We describe complex formation between a designed pentameric β-propeller and the anionic macrocycle sulfonato-calix[8]arene (sclx8), as characterized by X-ray crystallography and NMR spectroscopy. Each blade of this β-propeller is a 47-residue monomer of ∼5.2 kDa (yielding a pentamer of ∼26 kDa) that binds one equivalent of N-acetylglucosamine (GlcNAc). The Asn33Lys mutation makes the protein cationic, with a calculated isoelectric point, pI ∼ 8. As is typical of β-propellers, Pent has a toroidal structure with a funnel-like central channel.

The unusual crystals that grew in Tris-HCl at pH 8.8 diffracted to 1.7 Å resolution. These data were solved in space group P212121 with an asymmetric unit comprising one Pent. Despite the presence of 2 mM sclx8 during crystallization, there was no calixarene in this structure. This result can be interpreted in light of the crystallization pH, which is almost one unit above the calculated pI of Pent. Under these conditions, calixarene complexation is apparently switched off as the protein is anionic. This structure is further interesting as the crystal packing interfaces are distinct to those found in the Pent–sclx8 forms I and II. Furthermore, intramolecular noncovalent bonds such as the Lys5-Trp48 salt bridge are preserved in the Pent-only structure.

>[5x]MSGFKFLFFSPDGTLYGVHNDKLYKGTPPTSDKDNWLARATLIGNGGW{(3R,5R,6S)-5-(3-chlorophenyl)-6-(4-chlorophenyl)-1-[(1S)-1-cyclopropyl-2-(pyrrolidin-1-ylsulfonyl)ethyl]-3-methyl-2-oxopiperidin-3-yl}acetic 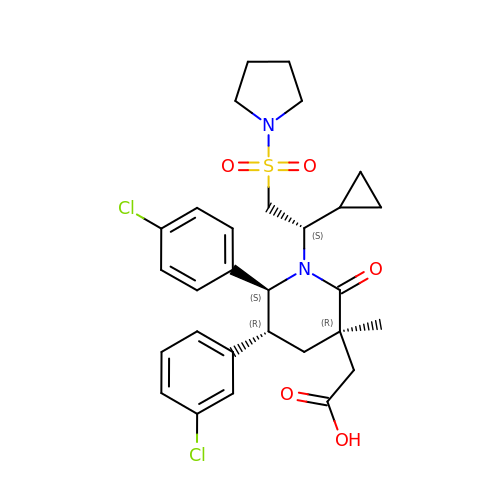acid | C29 H34 Cl2 N2 O5 S | JHVUPAFRBHMUAB-GCMXZSHTSA-N> SNAMDLSGKMVKQVEILSDGIVFYEIFRYRLYLISEMSPVNIQGVDLLEGNWGTVGSV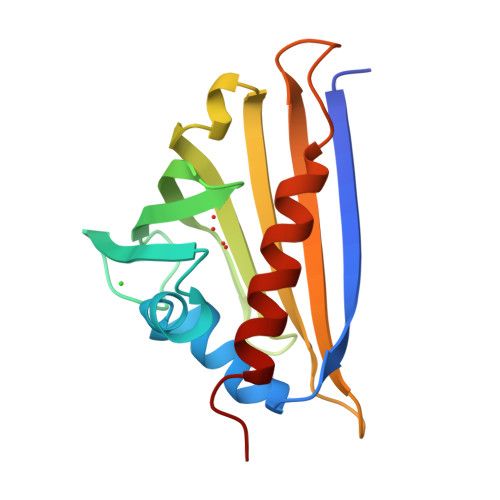IFFKYTIDGKEKTAKDIVEAIDEETKSVTFKIVEGDLMELYKTFIIIVQVDTKGEHNSVTWTFHYEKLKEDVEEPNTLMNFCIEITKDIETYHLK>MMSETAPLPSASSALEDKAASAPVVGIIMGSQSDWETMRHADALLTELEIPHETLIVSADRTPDRLADYARTAAERGLNVIIAGAGGAAHLPGMCAAWTRLPVLGVPVESRALKGMDSLLSIVQMPGG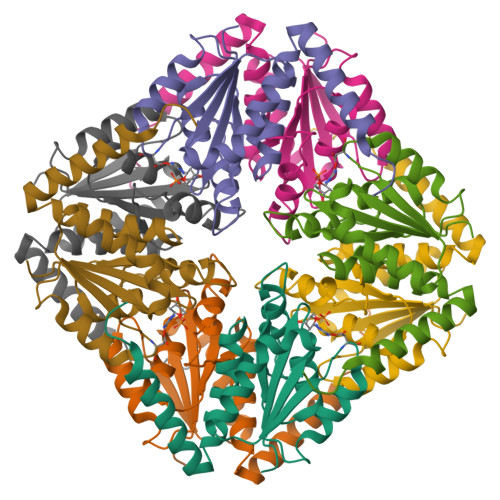VPVGTLAIGASGAKNAALLAASILALYNPALAARLETWRALQTASVPNSPITEDK[2x]> MNTATTVGVTGDGDARQRNSPEESEKRKRVSSAVQFLHDSRVKITPAANKIQFLKSKGLTTEEVCEAFEKAGQTIPLDEIKKIMNKPSFGQLGSGVVNNNLAPGHVGSDATYVLRQHPFMPHAGPLYTQQPPPFPQTPQGAKETDWRDVIIGVGAALISGFAAFKAFQIYSPYEIRRKDERTKKGS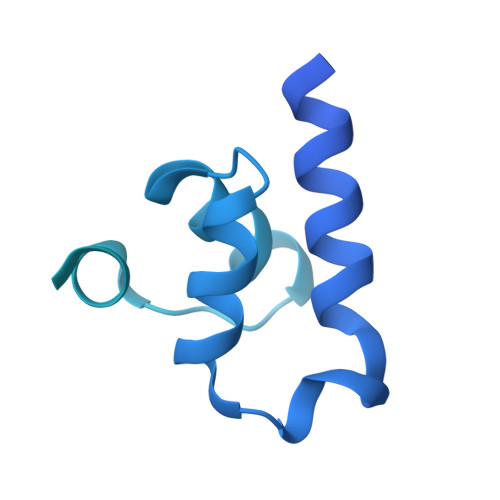RMESQRRGKRHEGSVSPDRGAERPVTSLHTMAPPMPATPTPLPTATAANAAESTEREIQKLQSELKETQEALEKEKRSKAEISVSLGKLRGQINALSRTNDNLESRIKLLQEEVDKANSEANKRKELDASFTGAADGVPKSQSEDAIQPNGPPLLTPKILADTVGCNSAALNELPVLTAVEFVPEE> IGDGYE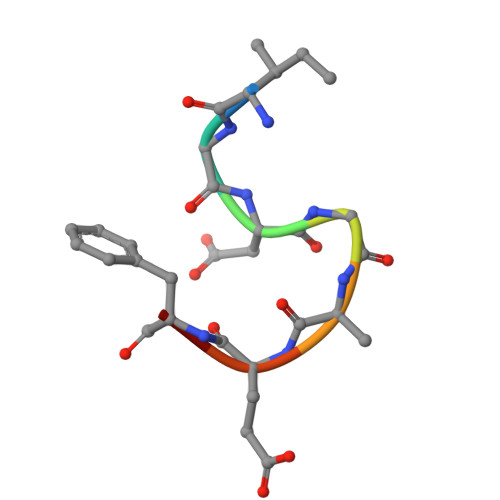FT>MRDPFMEALGLKVLHLAPGEAVVAGEVRADHLDLHGTAHGGFLYALADSAFALASNTRGPAVALSCRMDYFRPLGAGARVEAR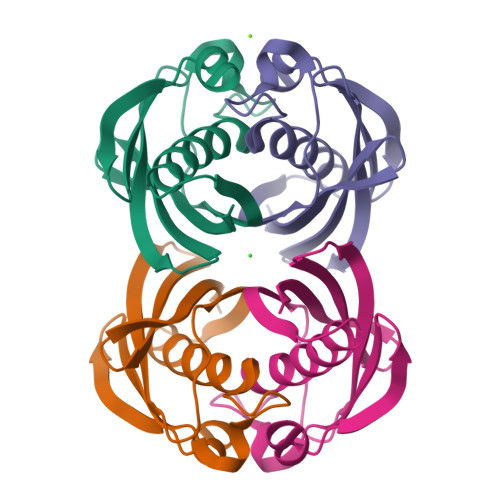AVEVNLSRRTATYRVEVVSEGKLVALFTGTVFRLGGDGDDVPAGTGNLAPREA[2x]> MIVSDIEANALLESVTKFHCGVIYDYSTAEYVSYRPSDFGAYLDALEAEVARGGLIVFHNGHKYDVPALTKLAKLQLNREFHLPRENCIDTLVLSRLIHSNLKDTD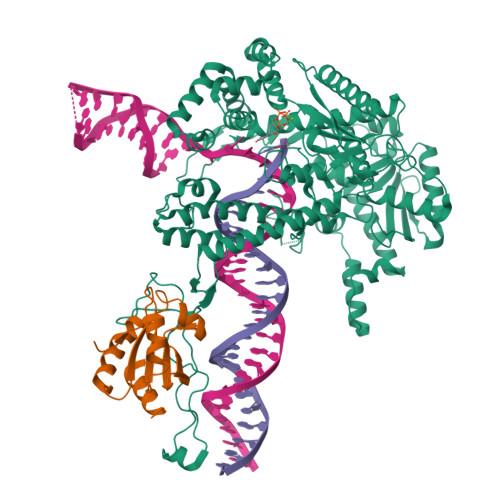MGLLRSGKLPGKRFGSHALEAWGYRLGEMKGEYKDDFKRMLEEQGEEYVDGMEWWNFNEEMMDYNVQDVVVTKALLEKLLSDKHYFPPEIDFTDVGYTTFWSESLEAVDIEHRAAWLLAKQERNGFPFDTKAIEELYVELAARRSELLRKLTETFGSWYQPKGGTEMFCHPRTGKPLPKYPRIKTPKVGGIFKKPKNKAQREGREPCELDTREYVAGAPYTPVEHVVFNPSSRDHIQKKLQEAGWVPTKYTDKGAPVVDDEVLEGVRVDDPEKQAAIDLIKEYLMIQKRIGQSAEGDKAWLRYVAEDGKIHGSVNPNGAVTGRATHAFPNLAQIPGVRSPYGEQCRAAFGAEHHLDGITGKPWVQAGIDASGLELRCLAHFMARFDNGEYAHEILNGDIHTKNQIAAELPTRDNAKTFIYGFLYGAGDEKIGQIVGAGKERGKELKKKFLENTPAIAALRESIQQTLVESSQWVAGEQQVKWKRRWIKGLDGRKVHVRSPHAALNTLLQSAGALICKLWIIKTEEMLVEKGLKHGWDGDFAYMAWVHDEIQVGCRTEEIAQVVIETAQEAMRWVGDHWNFRCLLDTEGKMGPNWAICH;> MSDKIIHLTDDSFDTDVLKADGAILVDFWAEWCGPCKMIAPILDEIADEYQGKLTVAKLNIDQNPGTAPKYGIRGIPTLLLFKNGEVAATKVGALSKGQLKEFLDANLA> ADVTITVNGK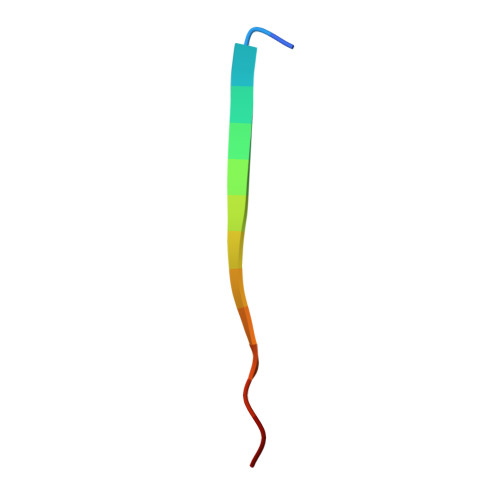VVAK> GPALAQDDVAPYFKTEPGLPQIHLEGNRLVLTCLAEGSWPLEFKWIRNDSELTTYSSEYKYIIPSLQKLDAGFYRCVVRNRMGALLQRKSEIQVAYMGNFMDTDQRKTVSQGHAALLNLLPIVSCPQPQVTWFREGHKIIPSSRIAITLENQLVILATTASDAGAYYVQAVNEKNGENKTSPFIHLSVARDTGTHEAMAPIIVVAPGNRSVVAGSSETTLECIANARPVEELSVHWKRNGVRLTSGLHSYGRRLTITNPTSADTGMYVCEATLRGSTFEPARARAFLSIIEPPYFTAEPESRILGEVEETMDIPCRAMGVPLPTLQWYKDAVPLSKLQNPRYKVLPSGGLHIQKLSPEDSGIFQCFASN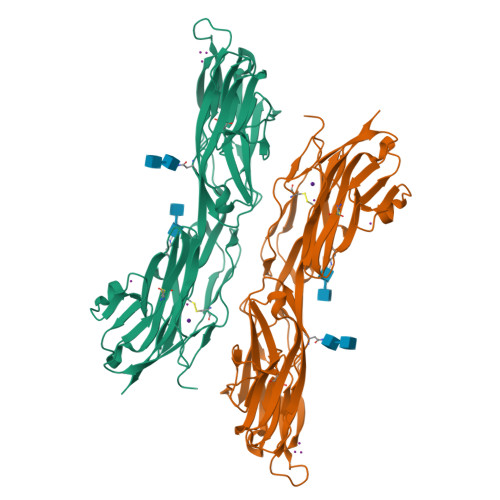EGGEVQTHTYLDVTN>[2x]MKTTYNRWWKKKVWFGRKDMSYKVIVDSCGEFTPEMKADGGFEHVALGIQIEDTQWTDDDSLKQEELLLKIAESTSCAKTSCPSPERYME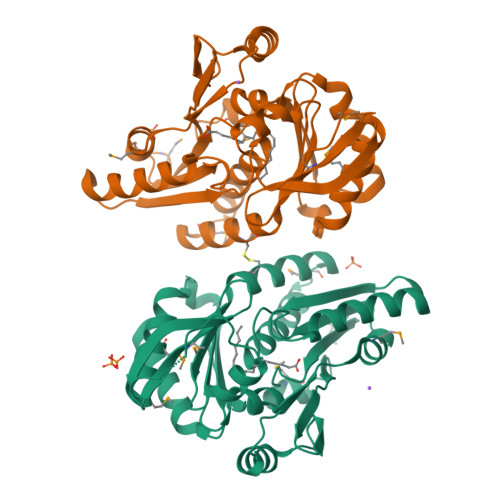SYHCDAERIYVVTLSAELSGSYNSAVLGKNLYEEEYGEKQIHVFNSRSASVGETLIALKVQQCEKAGMTFEEVVESVECYIEEQHTYFVLENLDTLRKNGRLTGIKSLVAGALNIKPIMGSTPQGTICQKEKARGMKKALVKMADCVAADVVNAGDKILAIAHCNCEERAKEVQRLLKERFAVKSSFIVDTSGISTVYANDGGIIVVV>MGELRVGLEESELWLRFKELTNEMIVTKNGRRMFPVLKVNVSGLDPNAMYSFLLDFVAADNHRWKYVNGEWVPGGKPEPQAPSCVYIHPDSPNFGAHWMKAPVSFSKVKLTNKLNGGGQIMLNSLHKYEPRIHIVRVGDPQRMITSHCFPETQFIAVTAYQNEEITALK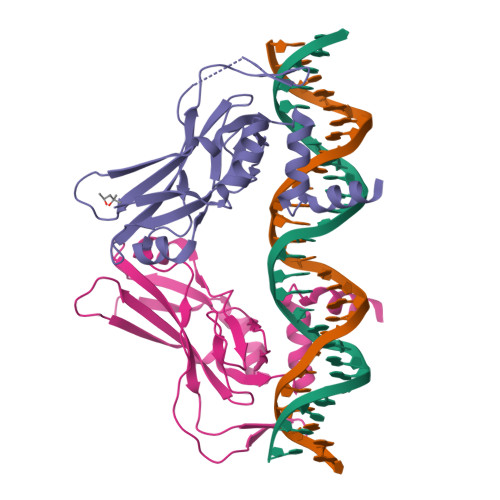IKYNPFAKAFLDAKERSHHHHHH[2x]(trimethylarsonio)acetate | C5 H11 As O2 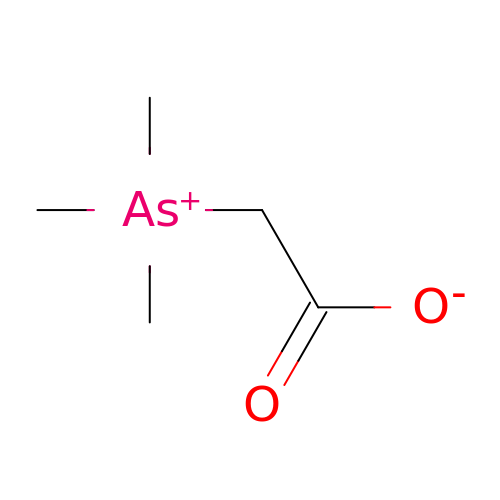| SPTHHTGLGVZZRH-UHFFFAOYSA-N>[2x]MAKSVPAIFLDRDGTINVDHGYVHEIDNFEFIDGVIDAMRELKKMGFALVVVTNQSGIARGK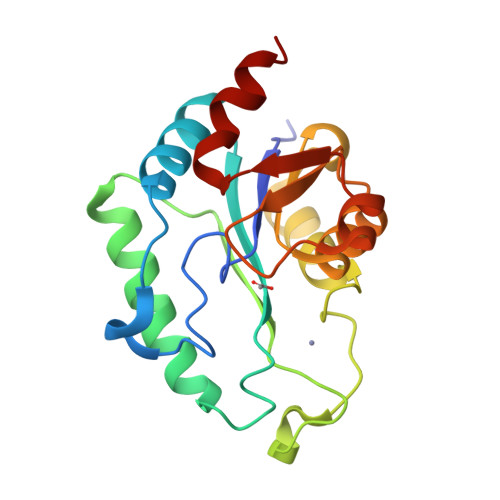FTEAQFETLTEWMDWSLADRDVDLDGIYYCPHHPQGSVEEFRQVCDCRKPHPGMLLSARDYLHIDMAASYMVGDKLEDMQAAVAANVGTKVLVRTGKPITPEAENAADWVLNSLADLPQAIKKQQ> SSQIRQNYSTEVEAAVNRLVNLYLRASYTYLSLGFYFDRDDVALEGVCHFFRFLAFFKLFGAFRLLKMQNQRGGRALFQDLQKPSQDEWGTTLDAMKAAIVLEKSLNQALLDLHALGSAQADPHLCDFLESHFLDEEVKLIKKMGDHLTNIQRLVGSQAGLGEYLFERLTLKHD

As a scaffold for aromatic cluster design, we chose ferritin as a protein cage platform with a 12 nm outer diameter and an 8 nm inner cavity, composed of 24 subunits. To prove this concept through protein engineering, we focused on a two‐fold symmetric inter‐subunit interface of a recombinant horse spleen apo‐L ferritin (Fr) as a target region for mutagenesis. Herein, we present the construction of an aromatic cluster with an artificial molecular binding pocket at the two‐fold symmetric interface of ferritin and explore its ligand‐binding characteristics. We developed a system that uses ligand binding as a driving force to induce and propagate changes in the orientation of multiple aromatic side chains.

To modulate the shape of the central pocket, we prepared Fr‐F5/59A (Fr‐E53F/E56F/E57F/R59A/E60F/E63F) and Fr‐F5/59L (Fr‐E53F/E56F/E57F/R59L/E60F/E63F) in which residue 59 was replaced with Ala or Leu (lower). Conversely, in Fr‐F5/59L, the introduction of leucine (Leu) imposes steric hindrance, effectively obstructing the pocket's entrance. These variances in pocket morphology among the variants are anticipated to impact ligand binding affinity and specificity. Replacing Phe59 with Ala or Leu significantly reduced the incorporation amount of NR (1.4 molecules for Fr‐F5/59A and 0.4 molecules for Fr‐F5/59L). In contrast, no electron density attributable to NR was observed in the difference Fourier map analysis of NR•Fr‐F5/59L, likely due to the entrance being blocked by L59 (distance between L59–L59' 4.1 Å), preventing NR entry due to steric hindrance.> HHHHDKNPGSENMTNTIGPHDRGGSSPIYNILNSYLTAYNGSHHLYDRMSFLCLSSQNTLNGACPSSDAPGTATIDGETNI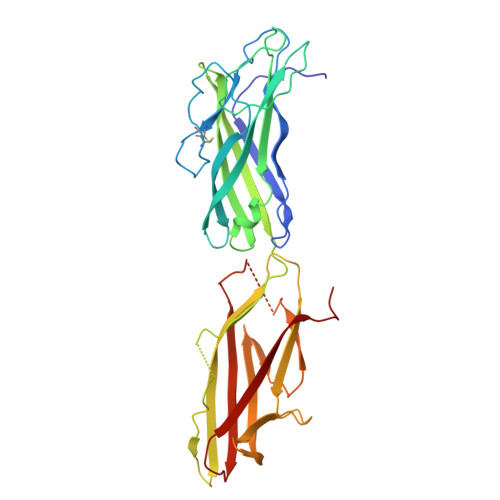TLQFTEKRSLIKRELQIKGYKQFLFKNANCPSKLALNSSHFQCNREQASGATLSLYIPAGELNKLPFGGVWNAVLKLNVKRRYDTTYGTYTINITVNLTDKGNIQIWLPQFKSNARVDLNLRPTGGGTYIGRNSVDMCFYDGYSTNSSSLEIRFQDDNSKSDGKFYLKKINDDSKELVYTLSLLLAGKNLTPTNGQALNINTASLETNWNRITAVTMPEISVPVLCWPGRLQLDAKVKNPEAGQYMGNIKITFTPSSQTL>[6x]MTKTVFHLGVTEADLNGATLAIIPGDPARVQKIAELMDNPVFLASHREYTVYRAELDGQSVVVCSTGIGGPSTSIAVEELAQLGVRTFLRVGTTGAIQPHVNVGDMIVTTGSVRLDGASLHFAPMEFPAVPDFDVATAMKAAAQESGATVHMGVTASSDTFYPGQERYDTFTGRVVRRFQGSMKEWQDMGVLNFEMESATLLTM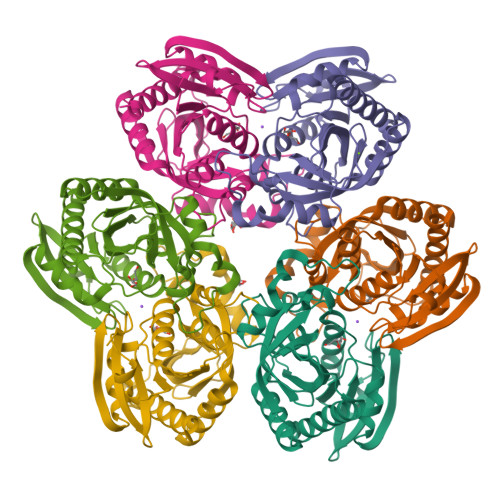CASSGLKAGCVAGVIINRTQKEIPDHATLKETEARSIKVVVEAARKMLK> PVATATATTVPATLAATTAAAATSFSTSAITISTSATPTNTTNNTFANEDSHRKCHRTRVEKVETPHVTIEDAQHRKPMDQKRSSSLGSNRSNRSHTSGRLRSPSNDSAHRSGDDQSGRKRVLHSGSRDREKTKSLEITGERKSRIDQLKRGEPSRSTSSDRQDSRSHSSRRSSPESDRQVHSRSGSFDSRDRLQERDRYEHDRERERERRDTRQREWDRDADKDWPRNRDRDRLRERERERERDKRRDLDRERERLISDSVERDRDRDRDRTFESSQIESVKRCEAKLEGEHERDLESTSRDSLALDKERMDKDLGSVQGFEETNKSERTESLEGDDESKLDDAHSLGSGAGEGYEPISDDELDEILAGDAEKREDQQDEEKMPDPLDVIDVDWSGLMPKHPKEPREPGAALLKFTPGAVMLRVGISKKLAGSELFAKVKETCQ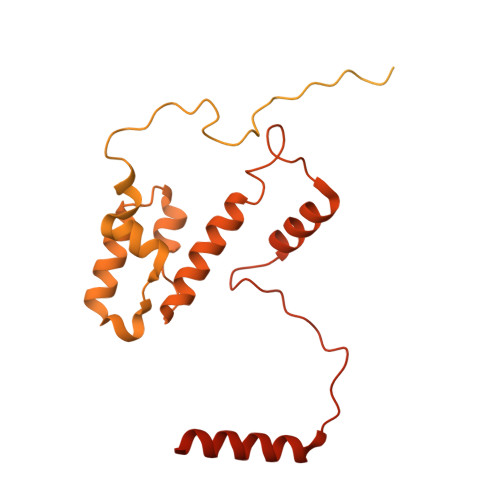RLLEKPKDADNLFEHELGALNMAALLRKEERASLLSNLGPCCKALCFRRDSAIRKQLVKNEKGTIKQAYTSAPMVDNELLRLSLRLFKRKTTCHAPGHEKTEDNKLSQSSIQQELCVS> GEVEWDAFSIPELQNFLTI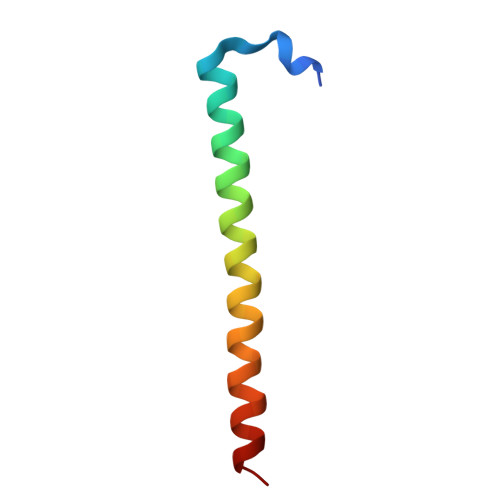LEKEEQDKIQQVQKKYDKFRQKLEEALRES>[2x]EPKLDMNKQKISPAEVAKHNKPDDCWVVINGYVYDLTRFLPNHPGGQDVIKFNAGKDVTAIFEPLHAPNVIDKYIAPEKKLGPLQGSMPPELVCPPYAPGETKEDIARKEQLKSLLPPLDNIINLYDFEYLASQTLTKQAWAYYSSGANDEVTHRENHNAYHRIFFKPKILVDVRKVDISTDMLGSHVDVPFYVSATALCKLGNPLEGEKDVARGCGQGVTKVPQMISTLASCSPEEIIEAAPSDKQIQWYQLYVNSDRKITDDLVKNVEKLGVKALFVTVDAPSLGQREKDMKLKFSNTKAGPKAMKKTNVEESQGASRALSKFIDPSLTWKDIEELKKKTKLPIVIKGVQRTEDVIKAAEIGVSGVVLSNHGGRQLDFSRAPIEVLAETMPILEQRNLKDKLEVFVDGGVRRGTDVLKALCLGAKGVGLGRPFLYANSCYGRNGVEKAIEILRDEIEMSMRLLGVTSIAELKPDLLDLSTLKARTVGVPNDVLYNEVYEGP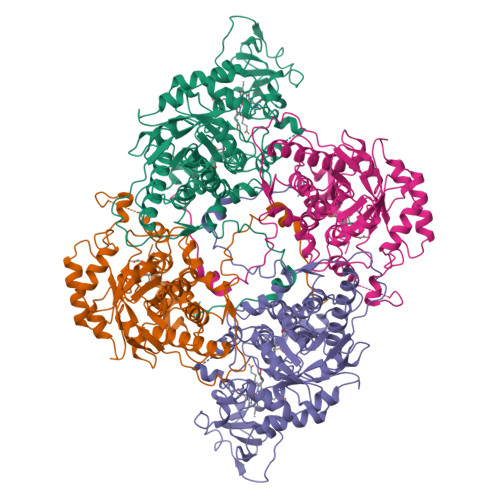TLTEFEDA> MLNYNAPIDGQKSSIDGAGSDQMNTFYWLKKAIIQARKDQYFMPLASVTNMPKNMGKTIKVYEYVPLLDDRNINDQGIDANGAHIVNGNLYGSSKDIGTITSKLPLLTENGGRVNRVGFTRLSREGSIHKFGF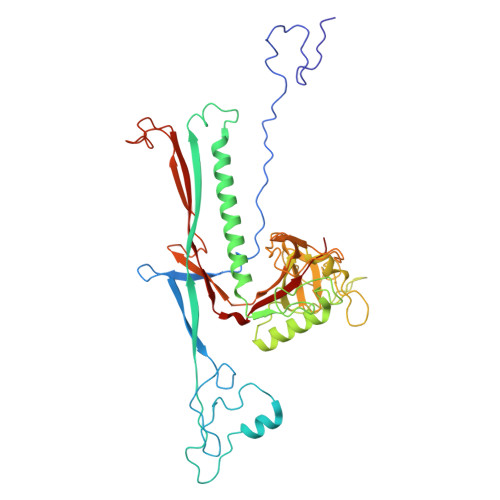FYEFTQESLDFDSDDQLKEHLSRELMNGAVQITEAVLQKDLLAAAGTVLYAGAATSDATITGEGSTPSVITYKNLMRLDAILTDNRTPTQTTIITGSRLVDTKVIGGTRVMYVGSELVPDLKAMKDLFGNKAFIEIQHYGDAGTLMNGEIGTIDKFRIIQVPEMLHWAGAGAAATDANPGYRTSTVNGTEHYDVYPVLVVGDDSFTTIGFQTDGKSVKFNVMTKMPGKETADRNDPYGETGFSSIKWYYGILVKRPERIAVMKAVAPL[(5R)-5-(5-METHYL-2,4-DIOXO-3,4-DIHYDROPYRIMIDIN-1(2H)-YL)-2,5-DIHYDROFURAN-2-YL]METHYL DIHYDROGEN PHOSPHATE 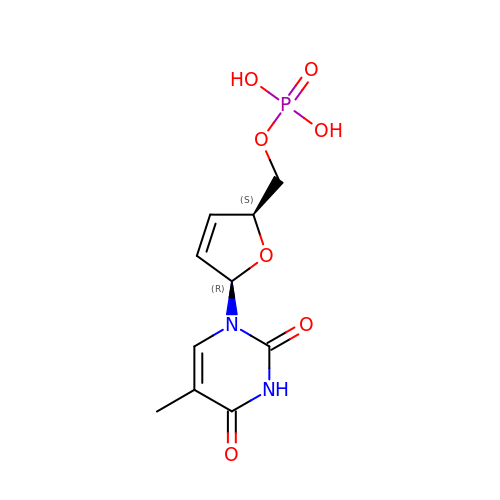| C10 H13 N2 O7 P | XLPGURCDSRIXFL-JGVFFNPUSA-N> VVNGIPTRTNIGWMVSLRYRNKHICGGSLIKESWVLTARQCFPSRDLKDYEAWLGIHDVHGRGDEKCKQVLNVSQLVYGPEGSDLVLMKLARPAVLDDFVSTIDLPNYGSTIPEKTSCSVYGWGYTGLINYDGLLRVAHLYIMGNEKCSQHHRGKVTLNESEICAGAEKIGSGPCEGDYGGPLVCEQHKMRMVLGVIVPGRGCAIPNRPGIFVRVAYYAKWIHKIILTYKVPQS;> ECKEALAKSEMNVNMKYQLPNFTAETPIQNVILHEHHIFLGATNYIYVLNEEDLQKVAEYKTGPVLEHPDCFPCQDCSSKANLSGGVWKDNINMALVVDTYYDDQLISCGSVNRGTCQRHVFPHNHTADIQSEVHCIFSPQIEEPSQCPDCVVSALGAKVLSSVKDRFINFFVGNTINSSYFPDHPLHSISVRRLKETKDGFMFLTDQSYIDVLPEFRDSYPIKYVHAFESNNFIYFLTVQRETLDAQTFHTRIIRFCSINSGLHSYMEMPLECILTELVPRGSTKKEVFNILQAAYVSKPGAQLARQIGASLNDDILFGVFAQSKPDSAEPMDRSAMCAFPIKYVNDFFNKIVNKNNVRCLQHFYGPNHEHCFNRTLLRNSSGCEARRDEYRTEFTTALQRVDLFMGQFSEVLLTSISTFIKGDLTIANLGTSEGRFMQVVVSRSGPSTPHVNFLLDSHPVSPEVIVEHTLNQNGYTLVITGKKITKIPLNGLGCRHFQSCSQCLSAPPFVQCGWCHDKCVRSEECLSGTWTQQICLP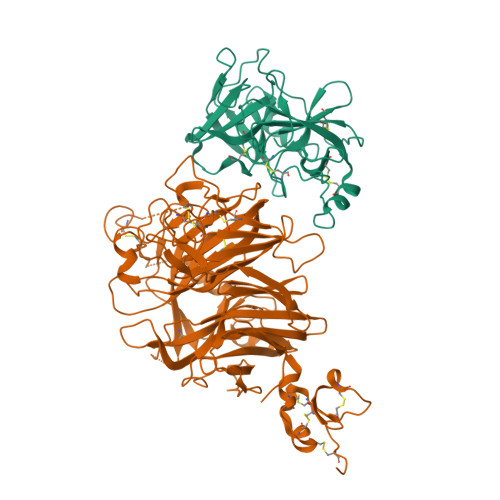AIYKHHHHHHHH>[2x]GPGSMSGIDPKRFGKVAVLFGGESAEREVSLTSGRLVLQGLRDAGIDAHPFDPAERPLSALKDEGFVRAFNALHGGYGENGQIQGALDFYGIRYTGSGVLGSALGLDKFRTKLVWQQTGVPTPPFETVMRGDDYAARATDIVAKLGLPLFVKPASEGSSVAVLKVKTADALPAALSEAATHDKIVIVEKSIEGGGEYTACIAGDLDLPLIKIVPAGEFYDYHA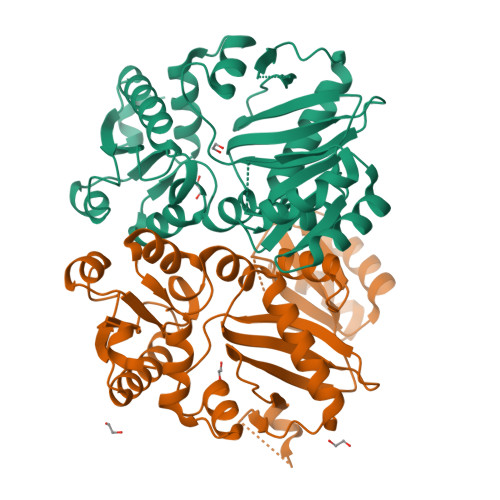KYVANDTQYLIPCGLPAEQETELKRIARRAFDVLGCTDWGRADFMLDAAGNAYFLEVNTAPGMTDHSLPPKAARSIGIGYSELVVKVLSLTLND> GSDELYRQSLEIISRYLREQATGAKDTKPMGRSGATSRKALETLRRVGDGVQRNHETAFQGMLRKLDIKNEDDVKSLSRVMIHVFSDGVTNWGRIVTLISFGAFVAKHLKTINQESCIEPLAESITDVLVRTKRDWLVKQRGWDGF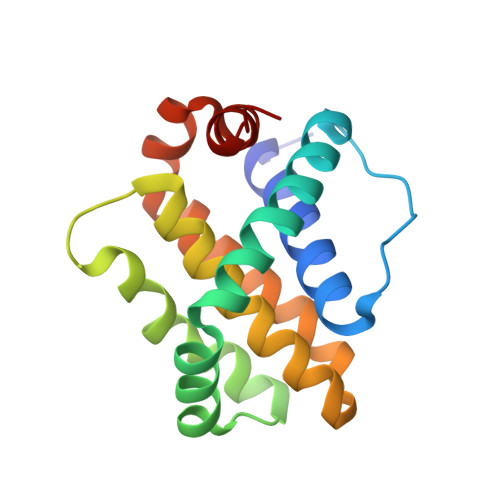VEFFHVED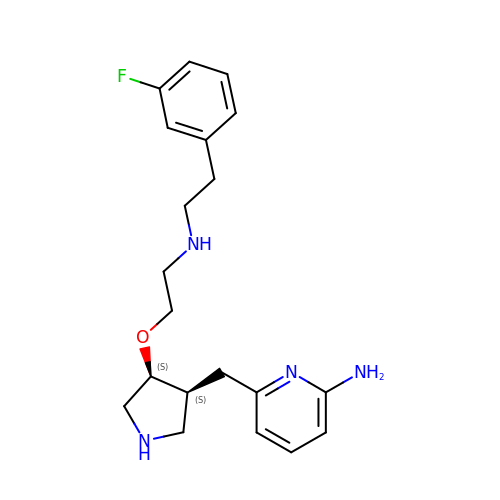6-{[(3S,4S)-4-(2-{[2-(3-fluorophenyl)ethyl]amino}ethoxy)pyrrolidin-3-yl]methyl}pyridin-2-amine | C20 H27 F N4 O | LRTPFJLYXDIXQR-QFBILLFUSA-N>ADPHHHHHHENLYFQGQKLDDVDPLVTTNFGKIRGIKKELNNEILGPVIQFLGVPYAAPPTGEHRFQPPEPPSPWSDIRNATQFAPVCPQNIIDGRLPEVMLPVWFTNNLDVVSSYVQDQSEDCLYLNIYVPTEDDIRDSGGPKPVMVYIHGGSYMEGTGNLYDGSVLASYGNVIVITVNYRLGVLGFLSTGDQAAKGNYGLLDLIQALRWTSENIGFFGGDPLRITVFGSGAGGSCVNLLTLSHYSEGLFQRAIAQSGTALSSWAVSFQPAKYARILATKVGCQVSDTVELVECLQKKPYKELVDQDVQPARYHIAFGPVIDGDVIPDDPQILMEQGEFLNYDIMLGVNQGEGLKFVENIVDSDDGVSASDFDFAVSNFVDNLYGYPEGKDVLRETIKFMYTDWADRHNPETRRKTLLALFTDHQWVAPAVATADLHSNFGSPTYFYAFYHHCQTDQVPAWADAAHGDEVPYVLGIPMIGPTELFPCNFSKNDVMLSAVVMTYWTNFAKTGDPNQPVPQDTKFIHTKPNRFEEVAWTRYSQKDQLYLHIGLKPRVKEHYRANKVNLWLELVPHLHN[2x];>[2x]HSAFAADPGHAGTTYIFSKGGGQITYKWPPNDRPSTRADRLAIGFSTVQKEAVLVRVDSSSGLGDYLELHIHQGKIGVKFNVGTDDIAIEESNAIINDGKYHVVRFTRSGGNATLQVDSWPVIERYPA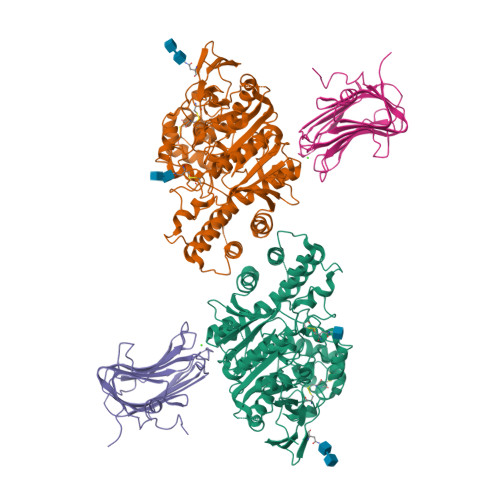GRQLTIFNSQATIIIGGKEQGQPFQGQLSGLYYNGLKVLNMAAENDANIAIVGNVRLVGEVPHHHHHHH4-[[(3S)-3-cyclopropyl-2-azaspiro[3.3]heptan-2-yl]methyl]-2-oxidanyl-N-[[(3R)-3-oxidanyl-1-[6-[(phenylmethyl)amino]pyrimidin-4-yl]piperidin-3-yl]methyl]benzamide 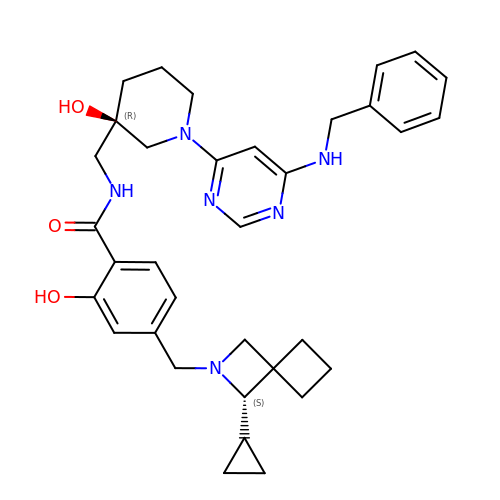| C34 H42 N6 O3 | SVGIQPUADMIIMK-AFPLUKJUSA-N> AEAGIT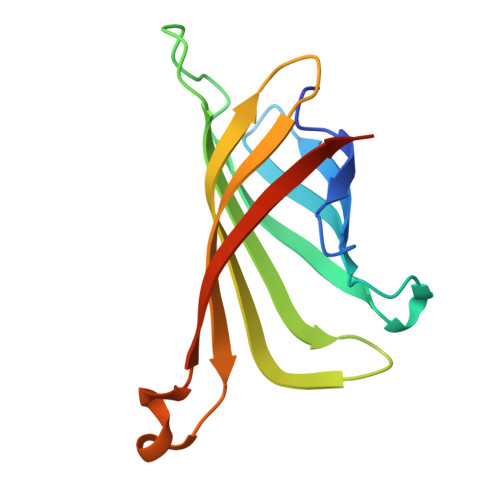GTWYAQLGDTFIVTAGADGALTGTYEAAVGNAESRYVLTGRYDSAPATDGSGTALGWTVAWKNNYRNAHSATTWSGQYVGGAEARINTQWLLTSGTTEANAWKSTLVGHDTFTKVKPSAASA>[2x]GQVAPNVWSKYFNIPNPGLRAYFSNVVSGQPEVYRTPFYKGMSLESICDEWYKKLVSIDTQWPTLMEFEDDLRKKVGPMSVMLPLKERMSDIDSYYDSISKDQVPFDTKAISAAKSEWKGVSRLRLRSEVNTVAVMKKSTNSGSPYFSKRKAVVSKTIPCDVYMDGRYCVMRQNGREWSGAAVLGWRGQEGGPKPTDVKQRVVWMFPFAVNIRELQVYQPLILTFQRLGLVPAWVSMEAVDRRITKMFDTKGPRDVVVCTDFSKFDQHFNPTCQSVAKELLADLLTGQEAVDWLERVFPIKYAIPLAYNWGEIRYGIHGMGSGS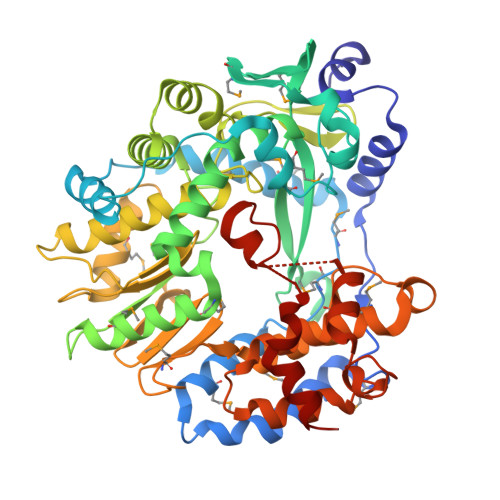GGTNADETLVHRVLQHEAAISHHTTLNPNSQCLGDDGVLTYPGISAEDVMQSYSRHGLDMNLEKQYVSKQDCTYLRRWHHTDYRVDGMCVGVYSTMRALGRLAMQERYYDPDVWGEKMVTLRYLSIIENVKYHPLKEEFLDFCIKGDKTRLGLGIPGFLDNIAGEAQKAIDMMPDFLGYTKSLQYDGDLRRNAAAGIENWWVVQALKSRR>ENDNYPIFTEETYTFTIFENCRVGTTVGQVCATDKDEPDTMHTRLKYSIIGQVPPSPTLFSMHPTTGVITTTSSQLDRELIDKYQLKIKVQDMDGQYFGLQTTSTCIINIDDVNDHLPTFTRTSYVTSVEENTVDVEILRVTVEDKDLVNTANWRANYTILKGNENGNFKIVTDAKTNEGVLCVVKPLNYEEKQQMILQIGVVNEAPFSREASPRSAMSTATVTVNVEDQDEGPECNPPIQTVRMKENAEVGTTSNGYKAYDPETRSSSGIRYKKLTDPTGWVTIDENTGSIKVFRSLDREAETIKNGIYNITVLASDQGGRTC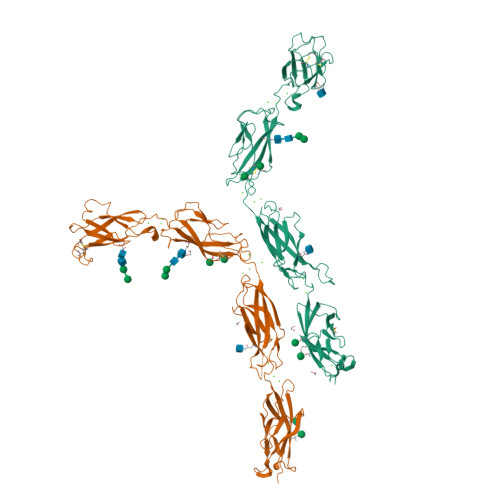TGTLGIILQDVNDNSPFIPKKTVIICKPTMSSAEIVAVDPDEPIHGPPFDFSLESSTSEVQRMWRLKAINDTAARLSYQNDPPFGSYVVPITVRDRLGMSSVTSLDVTLCDCITENDCTHRHHHHHH[2x]>GGGMDTLLILGDSLSAGYRMSAS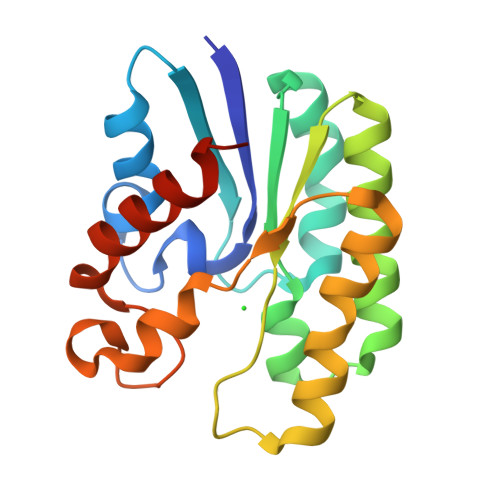AAWPALLNDKWQSKTSVVNASISGDTSQQGLARLPALLKQHQPRWVLVELGGNDGLRGFQPQQTEQTLRQILQDVKAANAEPLLMQIRLPANYGRRYNEAFSAIYPKLAKEFDVPLLPFFMEEVYLKPQWMQDDGIHPNRDAQPFIADWMAKQLQPLVNHDS[2x]> GPLGSKRQWTLEDFDIGRPLGKGKFGNVYLARERQSKFILALKVLFKTQLEKAGVEHQLRREVEIQSHLRHPNILRLYGYFHDATRVYLILEYAPLGTVYRELQKLSRFDEQRTATYITELANALSYCHSKRVIHRDIKPENLLLGSNGELKIADFGWSVHAPSSRRDTLCGTLDYLPPEMIEGRMHDEKVDLWSLGVLCYEFLVGMPPFEAHTYQETYRRISRVEFTFPDFVTEGARDLI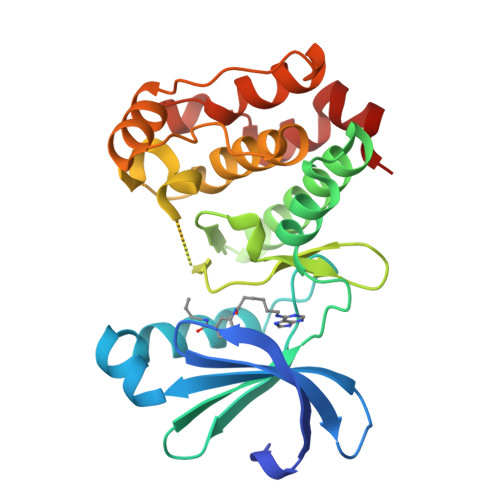SRLLKHNASQRLTLAEVLEHPWIKANSSKPS>MDYGMYFFEHVTPYETLVRRMERVIASGKTPFQDYFLFESKGFGKVLILDKDVQSTERDEYIYHETLVHPAMLTHPEPKRVLIVGGGEGAT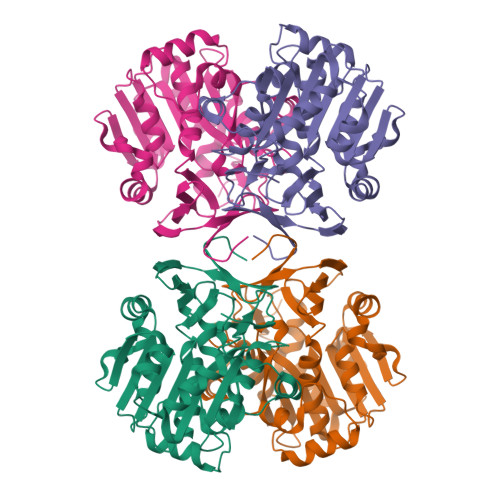LREVLKHPTVEKAVMVDIDGELVEVAKRHMPEWHQGAFDDPRAVLVIDDARAYLERTEERYDVVIIDLTDPVGEDNPARLLYTVEFYRLVKAHLNPGGVMGMQTGMILLTHHRVHPVVHRTVREAFRYVRSYKNHIPGFFLNFGFLLASDAFDPAAFSEGVIEARIRERNLALRHLTAPYLEAMFVLPKDLLEALEKETMVSTDQNPFYVTPEGEARQAPYKG[2x]>MTTLTRADWEQRAQNLKIEGRAFIQGEYTAAASGETFDCISPVDGRLLAKVASCDAADAQRAVESARSAFDSGAWSRLAPAKRKATMIRFAGLLEQNAEELALLETLDMGKPISDSLGVDIPGGARALSWSGEAIDKLYDEVAATPHDQLGLVTREPVGVVAAIVPWNFPLMMACWKLGPALSTGNSVVLKPSEKSPLTAIRIAQLAIEAGIPAGVLNVLPGYGHTVGKALALHMDVDTVVFTGSTKIAKQLMIYAGESNMKRVWLEAGGKSPNIVFADAPDLQAAADSAASAIAFNQGEVATAGSRLLVERSIKDRFLPM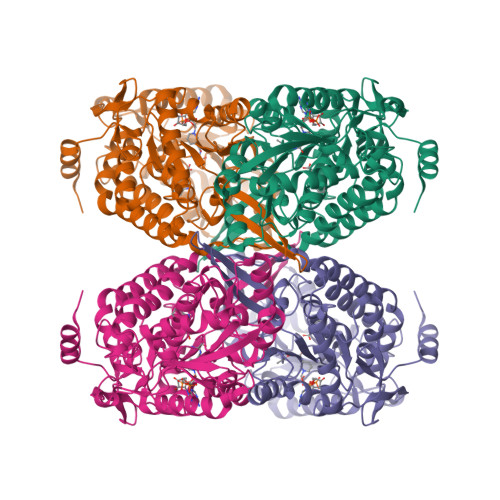VIEALGTWKPGNPLDPATNVGALVDTQQMNTVLSYIAAGHTDGARLVAGGKQILQETGGTYVEPTIFDGVNNAMRIAQEEIFGPVLSVLTFDTAEEAIQIANDTPYGLAAAVWTANLSKAHLTARALRAGSVWVNQYDGGDMTAPFGGFKQSGNGRDKSLHAFDKYTELKSTWIKL[8x]Tezacaftor | C26 H27 F3 N2 O6 | 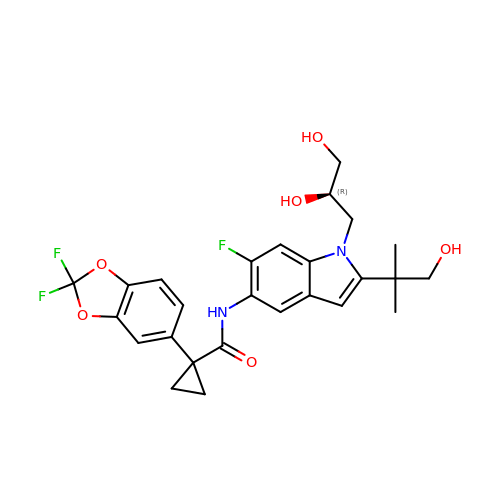MJUVRTYWUMPBTR-MRXNPFEDSA-N> ASSVNELENWSKWMQPIPDSIPLARISIPGTHDSGTFKLQNPIKQVWGMTQEYDFRYQMDHGARIFDIRGRLTDDNTIVLHHGPLYLYVTLHEFINEAKQFLKDNPSETIIMSLKKEYEDMKGAEDSFSSTFEKKYFVDPIFLKTEGNIKLGDARGKIVLLKRYSGSNEPGGYNNFYWPDNETFTTTVNQNANVTVQDKYKVSYDEKVKSIKDTMDETM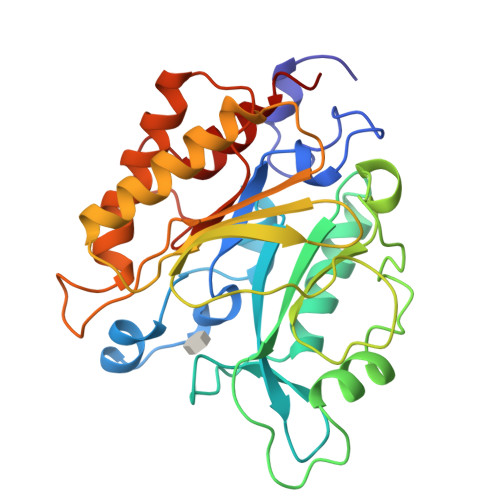NNSEDLNHLYINFTSLSSGGTAWNSPYYYASYINPEIANYIKQKNPARVGWVIQDYINEKWSPLLYQEVIRANKSLIKE>[2x]MATSLNTIDIQGDILVGMHKQKQLFYFFAINDPATFKTHLASDIAPVVASVTQLSNVATQPLVALNIAFSNTGLLALGVTDNLGDSLFANGQAKDATSFKESTSSWVPQFAGTGIHGVIILASDTTDLIDQQVASIESTFGSSISKLSSLSASIRPGNEAGHEMFGFLDGIAQPAINGFNTPLPGQNIVDAGVIITGATNDPITRPSWAVGGSFLAFRQLEQLVPEFNKYLLDNAPAGSGSLQARADLLGARMVGRWKSGAPIDLTPTADDPALGADAQRNNNFTYSHAGFDLGSDQSHCPFSAHIRKTRPRADLGGSLTPPNLSAGANSIMRSGIPYGPEVTSAESASNTTTQERGLAFVAYQAQLSQGFHFLQQTSADNANFPPGKTPATVGLDPIIGQNNGQPRVVNGLLPSNSSASLSIPQFVVSHGGEYFFSPPISAIGGRLSA

DyPs (dye-decolorizing peroxidases) (EC 1.11.1.19) represent a new family of haem peroxidases widespread in bacteria, archaea, fungi and other micro-organisms. In the present study, we expressed A. auricula-judae DyP in E. coli, solved the crystal structure of the recombinant enzyme and several site-directed variants, and used PELE (Protein Energy Landscape Exploration) to describe the binding of its typical substrate RB19. The DyP structure is formed by two domains, each of them including an antiparallel four-stranded large β-sheet and two or three helices resulting in a ferredoxin-like fold (plus two additional β-strands). In spite of the obvious similarity between the two domains, only the C-terminal domain harbours a haem cofactor.

Moreover, most of the variants show crystal structures largely superimposable with that of WT DyP, except for the mutated residues. Aromatic residues were changed to serine in the simple W377S, Y147S and Y337S variants (the latter with low refolding yield). The proof for Trp-377 being involved in the mixed protein radical was provided by the W377S variant. In the high-resolution narrow scan of its 9 GHz EPR spectrum (top), the tryptophanyl contribution observed for WT DyP completely disappeared (the spectrum of the W377S/Y147S variant, not shown, being nearly superimposable). As a main conclusion, Trp-377 appears responsible for the high-turnover catalytic site, since its substitution (W377S variant) completely prevented high-turnover oxidation of RB19 and DMP (and decreased over 40-fold the catalytic efficiency of high-turnover ABTS oxidation). In contrast, similar Tyr-337 and Tyr-147 variants (and the double Y147F/Y337F variant) only slightly affected substrate oxidation, and did not remove the high-turnover site.(1-methylpyrazol-4-yl)methyl 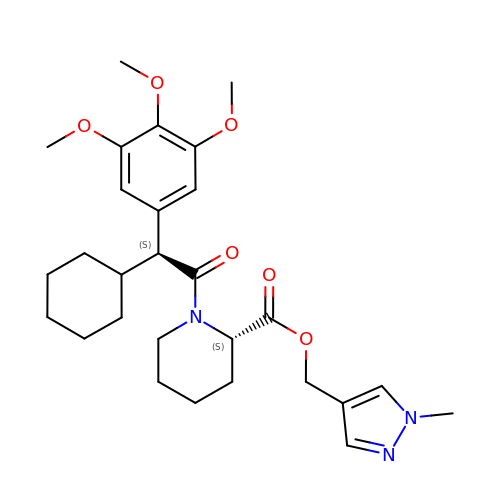(2S)-1-[(2S)-2-cyclohexyl-2-(3,4,5-trimethoxyphenyl)ethanoyl]piperidine-2-carboxylate | C28 H39 N3 O6 | AJBBOEPXPCJPNB-DHLKQENFSA-N> GHMRLPLDPTEFVRVLTGYLTGPRTAFHELVSAIAMVSRDSHDLQVAMDHFNRELMDGFSAHAAIIS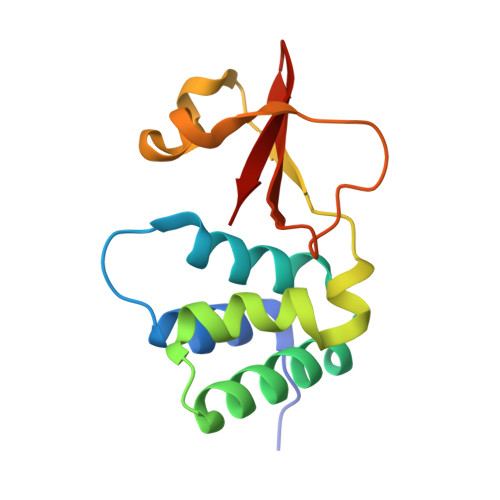ITQRCEYFRNCEAPTTQVTSKSQIPRAYHRRLRDVPEGPKTLGRGWVYIYLTPEGSLGLKI>[2x]MGSSMKLKHKRDDKMRFDIKKVLELAEKDFETAWRETRALIKDKHIDNKYPRLKPVYGKPHPVMETIERLRQAYLRMGFEEMINPVIVDEMEIYKQFGPEAMAVLDRCFYLAGLPRPDVGLGNEKVEIIKNLGIDIDEEKKERLREVLHLYKKGAIDGDDLVFEIAKALNVSNEMGLKVLETAFPEFKDLKPESTTLTLRSHMTSGWFITLSSLIKKRKLPLKLFSIDRCFRREQREDRSHLMSYHSASCVVVGEDVSVDDGKVVAEGLLAQFGFTKFKFKPDEKKSKYYTPETQTEVYAYHPKLGEWIEVATFGVYSPIALAKYNIDVPVMNLGLGVERLAMIIYGYEDVRAMVYPQFYEYRLSDRDIAGMIRVDKVPILDEFYNFANELIDICIANKDKESPCSVEVKREFNFNGERRVIKVEIFENEPNKKLLGPSVLNE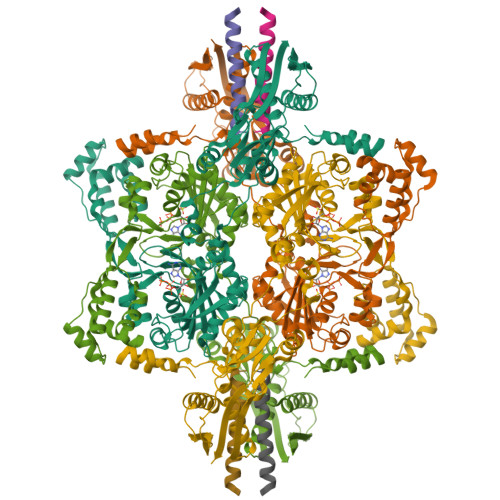VYVYDGNIYGIPPTFEGVKEQYIPILKKAKEEGVSTNIRYIDGIIYKLVAKIEEALVSNVDEFKFRVPIVRSLSDINLKIDELALKQIMGENKVIDVRGPVFLNAKVEIK;>MNHMRVEYSKDLIRKGISTISQLKKAKIRVEKDDKKISYKDAKPGKIDVNEFKKAIYLLIEADDFLYKKAPKHELNEEEAKEFCKLIIKCQEHLNKILANFGFEFEEKEIDEGALYIVSNKKLFKKLKNKNPNLKVVCTEGMLDIEDMRAIGVPEKALEGLKKKVEIARKNVERFIEKYKPEKIFVVVEDDKDELLYLRAKNLYNAEKLDADEILD[2x]>[6x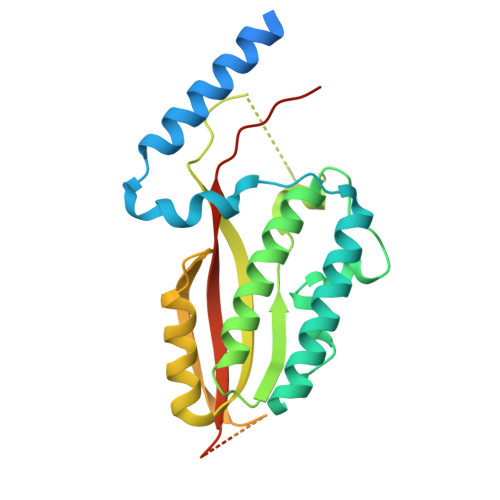]MIVNSKRSELDKKISIAAKEIKSANAAEITPSRSSNEELEKELNRYAKAVGSLETAYKPFLASSALVPTTPTAFQNELKTFRDSLISSCKKKNILITDTSSWLGFQVYSTQAPSVQAASTLGFELKAINSLVNKLAECGLSKFIKVYRPQLPIETPANNPEESDEADQAPWTPMPLEIAFQGDRESVLKAMNAITGMQDYLFTVNSIRIRNERMMPPPIANPAAAKPAAAQPATGAASLTPADEAAAPAAPAIQQVIKPYMGKEQVFVQVSLNLVHFNQPKAQEPSEDLEHHHHHH> SNAVELLQVDADLQAEIVGKYNADLQKAVQIEEKKASEIATEAVKEHVTAEYEERYAEHEEHDRI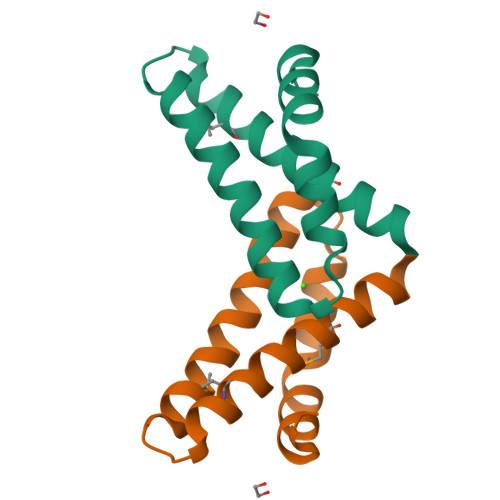MRDVAEILEQMEHAEVRRLITEDKVRPD> MAGPVSLRDLLMGASAWMGSESPGGSPTEGGGSAAGGPEPPWREDEICVVGIFGKTALRLNSEKFSLVNTVCDRQVFPLFRHQDPGDPGPGIRTEAGAVGEAGGAEDPGAAAGGSVRGSGAVAEGNRTEAGSQDYSLLQAYYSQESKVLYLLLTSICDNSQLLRACRALQSGEAGGGLSLPHAEAHEFWKHQEKLQCLSLLYLFSVCHILLLVHPTCSFDITYDRVFRALDGLRQKVLPLLKTAIKDCPVGKDWKLNCRPCPPRLLFLFQLNGALKVEPPRNQDPAHPDKPKKHSPKRRLQHALEDQIYRIFRKSRVLTNQSINCLFTVPANQAFVYIVPGSQEEDPVGMLLDQLRSHCTVKDPESLLVPAPLSGPRRYQVMRQHSRQQLSFHIDSSSSSSSGQLVDFTLREFLWQHVELVL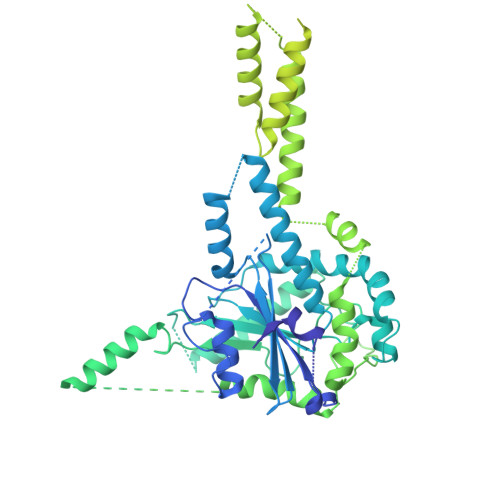SKKGFDDSVGRNPQPSHFELPTYQKWISAASKLYEVAIDGKEEDLGSPTGELTSKILSSIKVLEGFLDIDTKFSENRCQKALPMAHSAYQSNLPHNYTMTVHKNQLAQALRVYSQHARGPAFHKYAMQLHEDCYKFWSNGHQLCEERSLTDQHCVHKFHSLPKSGEKPEADRNPPVLYHNSRARSTGACNCGRKQAPRDDPFDIKAANYDFYQLLEEKCCGKLDHINFPVFEPSTPDPAPAKNESSPAPPDSDADKLKEKEPQTQGESTSLSLALSLGQSTDSLGTYPADPQAGGDNPEVHGQVEVKTEKRPNFVDRQASTVEYLPGMLHSNCPKGLLPKFSSWSLVKLGPAKSYNFHTGLDQQGFIPGTNYLMPWDIVIRTRAEDEGDLDTNSWPAPNKAIPGKRSAVVMGRGRRRDDIARAFVGFEYEDSRGRRFMCSGPDKVMKVMGSGPKESALKALNSDMPLYILSSSQGRGLKPHYAQLMRLFVVVPDAPLQIILMPQVQPGPPPCPVFYPEKQEITLPPDGLWVLRFPYAYVTERGPCFPPKENVQLMSYKVLRGVLKAVTQ6-(hydroxymethyl)[2,2'-bipyridin]-4-ol | C11 H10 N2 O2 | 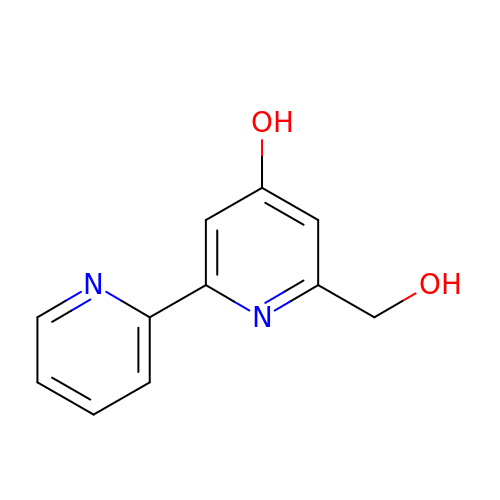HKHZGZONLACWBE-UHFFFAOYSA-N> MAQILPIRFQEHLQLQNLGINPANIGFSTLTMESDKFICIREKVGEQAQVVIIDMNDPSNPIRRPISADSAIMNPASKVIALKAGKTLQIFNIEMKSKMKAHTMTD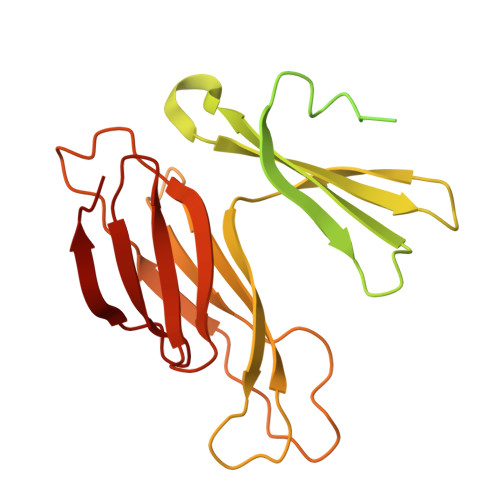DVTFWKWISLNTVALVTDNAVYHWSMEGESQPVKMFDRHSSLAGCQIINYRTDAKQKWLLLTGISAQQNRVVGAMQLYSVDRKVSQPIEGHAASFAQFKMEGNAEESTLFCFAVRGQAGGKLHIIEVGTPPTGNQPFPKKAVDVFFPPEAQNDFPVAMQISEKHDVVFLITKYGYIHLYDLETGTCIYMNRIS>MPFSDFVLALKDNPYFGAGFGLVGVGTALAMARKGAQLGLVAFRRHYMITLEVPARDRSYAWLLSWLTRHSTRTQHLSVETSYLQHESGRISTKFEFIPSPGNHFIWYQGKWIRVERNRDMQMVDLQTGTPWESVTFTALGTDRKVFFNILEEARALALQQEEGKTVMYTAVGSEWRTFGYPRRRRPLDSVVLQQGLADRIVKDIREFIDNPKWYIDRGIPYRRGYLLYGPPGCGKSSFITALAGELEHSICLLSLTDSSLSDDRLNHLLSVAPQQSLVLLEDVDAAFLSRDLAVENPIKYQGLGRLTFSGLLNALDGVASTEARIVFMTTNYIDRLDPALIRPGRVDLKEYVGYCSHWQLTQMFQRFYPGQAPSLAENFAEHVLKATSEISPAQVQGYFMLYKNDPMGAVHNIESLRHHHHHH[7x]

The human AAA-ATPase Bcs1L translocates the fully assembled Rieske iron-sulfur protein (ISP) precursor across the mitochondrial inner membrane, enabling respiratory Complex III assembly. Bcs1L is a membrane-bound oligomer, with each subunit consisting of an N-terminal TM segment, a middle Bcs1-specific domain, and a C-terminal AAA domain that is highly distinct, forming a clade of its own in the broad AAA protein family. Here, we captured Bcs1L conformations by cryo-EM during active ATP hydrolysis in the presence or absence of ISP substrate. In contrast to the threading mechanism widely employed by AAA proteins in substrate translocation, subunits of Bcs1L alternate uniformly between ATP and ADP conformations without detectable intermediates that have different, co-existing nucleotide states, indicating that the subunits act in concert.

Previously, we reported the structure of mBcs1L in the absence of nucleotide and substrate (Apo mBcs1L) determined by cryo-EM with imposed C7 symmetry. When we imposed no symmetry (C1) in reprocessing this data set, the resulting EM map at 4.4 Å resolution showed significant asymmetrical arrangement of mBcs1L subunits in the AAA ATPase domain with appearance of large crevices between some subunits. Inspections of the model built into the map confirmed that the separations between neighboring subunits in the AAA domains are not uniform. In particular, the separation between subunits A and G is clearly wider than others. This asymmetry is also reflected in the rms deviation of 1.222 Å for 2,259 residues when the C1 model is superposed to the C7 model, which is rather large compared to those identically calculated with the ATP- and ADP-bound structures of 0.285 Å and 0.248 Å, respectively. The apparent weak AAA domain association of mBcs1L subunits in the apo state is supported by the calculated buried surface area (BSA) between pairs of neighboring subunits, with lower BSA indicating weaker associations. In particular, the BSA between subunits A and G is the smallest at 4317 Å2. Calculations of BSA for ADP- and ATP-bound mBcs1L showed on average ~1000 Å2 more buried surface area than that for apo mBcs1L, suggesting that nucleotide binding stabilizes oligomeric states. Furthermore, the structure of Apo mBcs1L, when reconstructed without imposed symmetry, displays asymmetric arrangement of subunits, suggesting a potential mechanism for substrate ISP precursor release. Bcs1 subunits in apo state show significant asymmetric arrangement with large gaps between some subunits and are more prone to dissociate, which implies a mechanism for ISP precursor release, where Bcs1 subunits open up laterally in apo state to let ISP precursor diffuse out.N-{(3R,4S)-4-[(6-amino-4-methylpyridin-2-yl)methyl]pyrrolidin-3-yl}-N'-[2-(3-fluorophenyl)ethyl]ethane-1,2-diamine 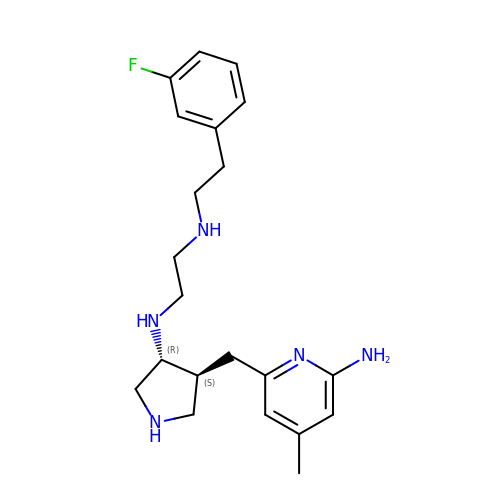| C21 H30 F N5 | PUOKPLCASUFBAN-PXNSSMCTSA-N> AAPTAYTPLDVAQAYQFPEGLDGQGQCIAIIELGGGYDETSLAQYFASLGVSAPQVVSVSVDGATNQPTGDPNGPDGEVELDIEVAGALAPGAKIAVYFAPNTDAGFLNAITTAVHDPTHKPSIVSISWGGPEDSWAPASIAAMNRAFLDAAALGVTVLAAAGDSGSTDGEQDGLYHVDFPAASPYVLACGGTRLVASAGRIERETVWNDGPDGGSTGGGVSRIFPLPSWQERANVPPSANPGAGSGRGVP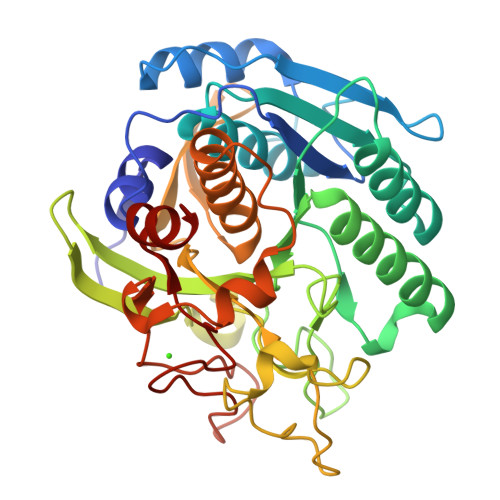DVAGNADPATGYEVVIDGETTVIGGTSAVAPLFAALVARINQKLGKPVGYLNPTLYQLPPEVFHDITEGNNDIANRARIYQAGPGWDPCTGLGSPIGIRLLQALLP>MSCYIYWDKIKRIASRLEGMNYHFDEMDTSGVMPLLDEIEEIAHDSTIDFESAKHILDDAEMNHALSLIRKFYVNLGMKLEMEKAQEVIESDSPWETLRSFYFYPRYLELLKNEAALGRFRRGERAVFIGGGPLPLTGILLSHVYGMRVNVVEIEPDIAELSRKVIEGLGVDGVN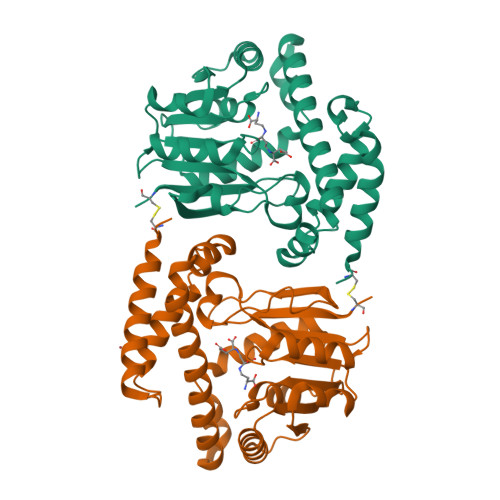VITGDETVIDGLEFDVLMVAALAEPKRRVFRNIHRYVDTETRIIYRTYTGMRAILYAPVSDDDITGFRRAGVVLPSGKVNNTSVLVFKCPDKGELNSKLEGKPIPNPLLGLDSTRTGHHHHHH[2x]>TGSKPFTVPILTVEEMTNSRFPIPLEKLFTGPSGAFVVQPQNGRCTTDGVLLGTTQLSPVNICTFRGDVTHIAGSRNYTMNLASLNWNNYDPTEEIPAPLGTPDFVGKIQGLLTQTTKGDGSTRGHKATVYTGSAPFTPKLGSVQFSTDTENDFETHQNTKFTPVGVIQDGSTTHRNEPQQWVLPSYSGRNVHNVHLAPAVAPTFPGEQLLFFRSTMPGCSGYPNMDLDCLLPQEWVQHFYQEAAPAQSDVALLRFVNPDTGRVLFECKLHKSGYVTVAHTGQHDLVIPPNGYFRFDSWVNQFYTLAP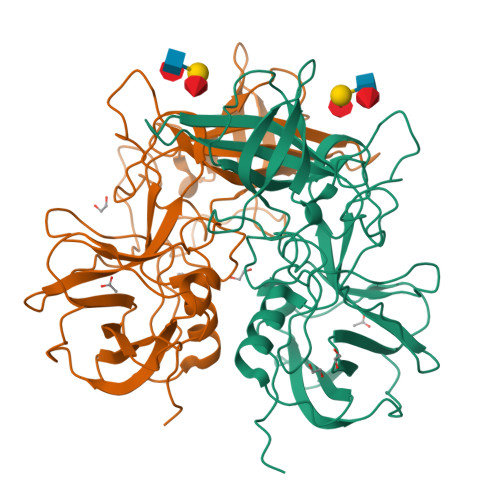M[2x]>MNPNQKIITIGSVSLTIATVCFLMQIAILATTVTLHFKQHECDSPASNQVMPCEPIIIERNITEIVYLNNTTIEKEICPKVVEYRNWSKPQCQITGFAPFSKDNSIRLSAGGDIWVTREPYVSCDPGKCYQFALGQGTTLDNKHSNDTVHDRIPHRTLLMNELGVPFHLGTRQVCIAWSSSSCHDGKAWLHVCITGDDKNATASFIYDGRLVDSIGSWSQNILRTQESECVCINGTCTVVMTDGSASGRADTRILFIEEGKIVHISPLSGSAQHIEECSCYPRYPGVRCICRDNWKGSNRPVVDINMEDYSIDSSYVCSGLVGDTPRNDDSSSNSNCRNPNNERGTQGVKGWAFDNGNDLWMGRTISKESRSGYETFKVIGGWSTPNSKSQVNRQVIV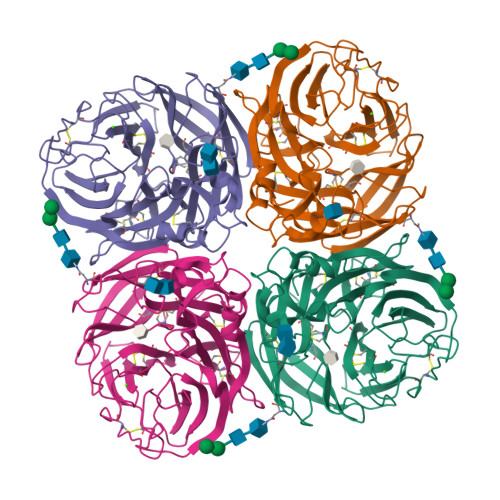DNNNWSGYSGIFSVEGKSCINRCFYVELIRGRPQETRVWWTSNSIVVFCGTSGTYGTGSWPDGANINFMPI[4x]DEOXY-GALACTO-NOEUROSTEGINE | C8 H15 N O3 | 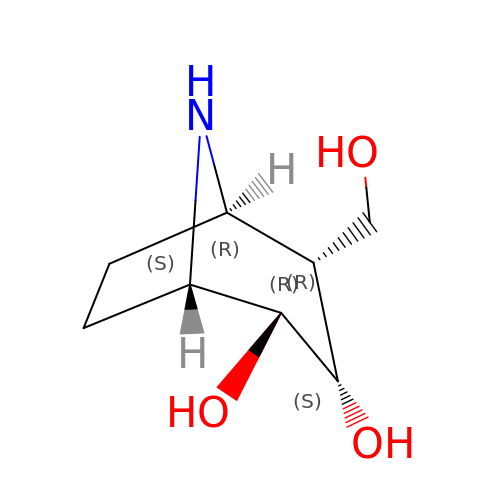GQKYZJDPLYFSSX-GWVFRZDISA-N Bacterial HSS is mostly found in α-proteobacteria and in some β- and γ-proteobacteria, including pathogenic strains such as Legionella pneumophila, Brucella spp. and various P. aeruginosa strains, including PA7 and PA14. It catalyzes the conversion of two molecules of putrescine (PUT; 1,4-diaminobutane) into one molecule of sym-homospermidine [HSP; bis(4-aminobutyl)amine] as the main reaction along with several side reactions (Ober et al., 1996; Böttcher et al., 1994). Bacterial HSS is NAD+-dependent, active at neutral to basic pH with an optimum at pH ∼8.8, and shows increased activity in the presence of 50 mM potassium ion. BvHSS forms a dimer, with each subunit containing a boot-shaped substrate-binding pocket between an NAD(P)-binding Rossmann-like domain and an HSS-like domain. The cofactor NAD+ is bound as a prosthetic group in the binding pocket with its nicotinamide ring being part of the active site.

The reaction mechanism of the nicotinamide adenine dinucleotide (NAD+)-dependent bacterial HSS has previously been characterized based on crystal structures of Blastochloris viridis HSS (BvHSS). This study presents the crystal structure of P. aeruginosa HSS (PaHSS) in complex with its substrate putrescine. The PaHSS structure was solved in space group P3212 using the Phaser tool implemented in Phenix and allowing both enantiomorphic space groups as possible solutions. Six PaHSS molecules were modeled into the asymmetric unit and refined to a maximum resolution of 2.42 Å. All six PaHSS molecules contain an NAD+ molecule in their binding pockets, and molecules A, C and E additionally contain a PUT molecule in the active site. We assume it to originate from the expression host and to be co-purified within the active site of PaHSS. The ‘inner’ and ‘outer’ amino groups of the PUT molecules form salt bridges with the carboxyl O atoms of Glu206 and Glu233, respectively, with distances of between 2.8 and 3.2 Å. Although PaHSS was shown to be a monomer in solution by SEC-MALS (the theoretical molecular weight of the monomer and the estimated molecular weight according to HPLC-MALS were 52 kDa; data not shown), these interface areas indicate the formation of three crystalline dimers by the six protein molecules within the asymmetric unit. The NAD+ molecules similarly insert their nicotinamide rings into the active site of the binding pockets, albeit with a slight offset. In addition, the ‘track-and-trace’ loop and particularly α-helix J of PaHSS are shifted in relation to BvHSS, providing more space for the pocket entrance compared with the BvHSS structure. However, the geometry in PaHSS is less favorable and the interaction energies are thus assumed to be weaker than in BvHSS. In conclusion, this inferior cation–π interaction geometry in PaHSS might be the reason for its reduced activity compared with BvHSS (see below).

>[6x]GPMDFSINPPQRIVFVGLGTIAQSFLPLLSKVHDLSTLEIYAIDPKTPPLIEYFANSFGLKFINSAIDQINYRDILVPILGEGTVLINLSTDVSSLALIELCRSAGALYLDTCIEPWKGGYDDPTIPLHKRTNYHLREQMLSLKKRLGSGVTALVAHGANPGLVSHFVKRALLDLAEEILGDCKKPSNKEQWAILSQRLGVKVIHVAEYDSQISQKSRERGEFVNTWSVHGFISESQQPAELGWGSHERSLPTDASMHTDGCGAAIYIEKPGASVRVKTWTPFNGPSLGYLVTHHEAISIADFLTLRTADETYRPTVHYAYRPSDEAILSVHEWFGNDCMTPEKTKVLRPGDILSGSDYLGVLLMGHEKSSYWYGSILSIEKAKELATLNTATTLQVAAGVLSGYLWILSHPSAGIIEAEDMDHEVALSYISQYLGELKGVYSDWNPTKNNPGTFSAIDSDSPWLFSNFVL>[2x]MEDLALRPKTLDEYIGQERLKQKLRVYLEAAKARKEPLEHLLLFGPPGLGKTTLAHVIAHELGVNLRVTSGPAIEKPGDLAAILANSLE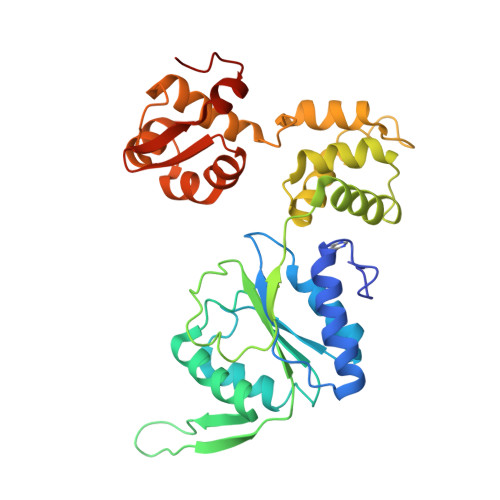EGDILFIDEIHRLSRQAEEHLYPAMEDFVMDIVIGQGPAARTIRLELPRFTLIGATTRPGLITAPLLSRFGIVEHLEYYTPEELAQGVMRDARLLGVRITEEAALEIGRRSRGTMRVAKRLFRRVRDFAQVAGEEVITRERALEALAALGLDELGLEKRDREILEVLILRFGGGPVGLATLATALSEDPGTLEEVHEPYLIRQGLLKRTPRGRVPTELAYRHLGYPPPVGPLLEP>[2x]GHMGITAIALYDYQAAGDDEISFDPDDIITNIEMIDDGW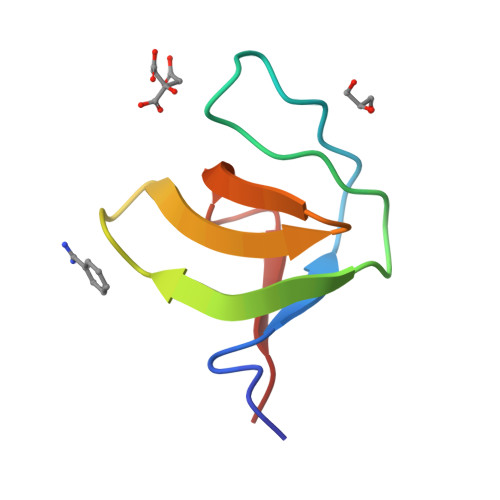WRGVCKGRYGLFPANYVELRQ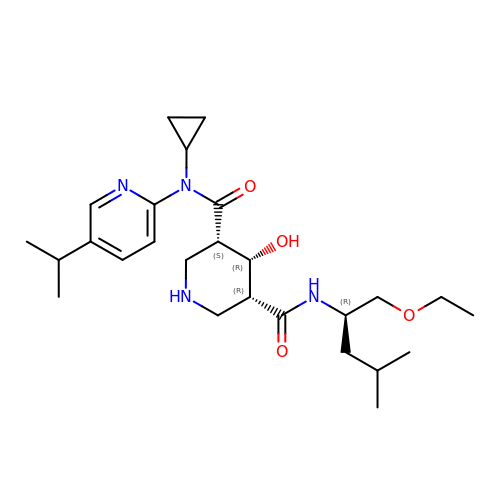(3S,4R,5R)-N-cyclopropyl-N'-[(2R)-1-ethoxy-4-methylpentan-2-yl]-4-hydroxy-N-[5-(propan-2-yl)pyridin-2-yl]piperidine-3,5-dicarboxamide | C26 H42 N4 O4 | YOVGCKBDPOHLAV-CNIHBODFSA-N>[2x]MSEDPILT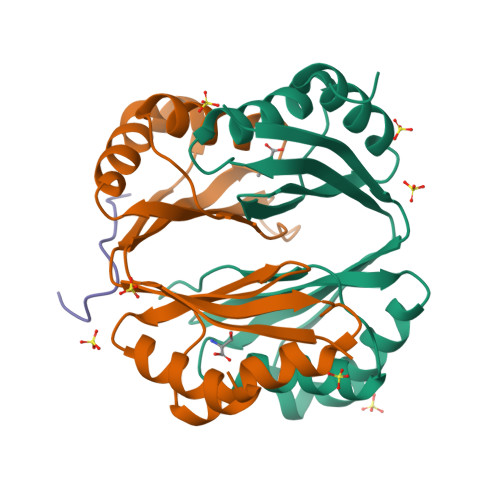GVAHDRSEAKVTIVGLPDIPGYAAKVFRAVADADVNIDMVLQNVSKVEDGKTDITFTCSRDVGPAAVEKLDSLRNEIGFSQLLYDDHIGKVSLIGAGMRSHPGVTATFCEALAAVGVNIELISTSEIRISVLCRDTELDKAVVALHEAFGLGGDEEATVYAGTGRLEHHHHHH;> EATVYAGTGRL> G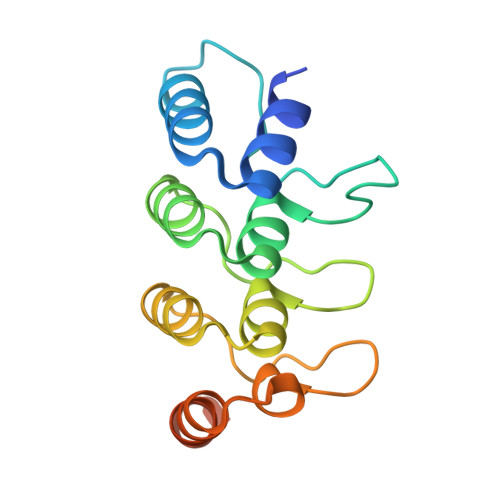SAMGSAEQQLLHHARNGNAEEVRQLLETMARNEVIADINCKGRSKSNLGWTPLHLACYFGHRQVVQDLLKAGAEVNVLNDMGDTPLHRAAFTGRKELVMLLLEYNADTTIVNGSGQTAKEVTHAEEIRSMLEAVERTQQRKLEELLLAAAREG>[8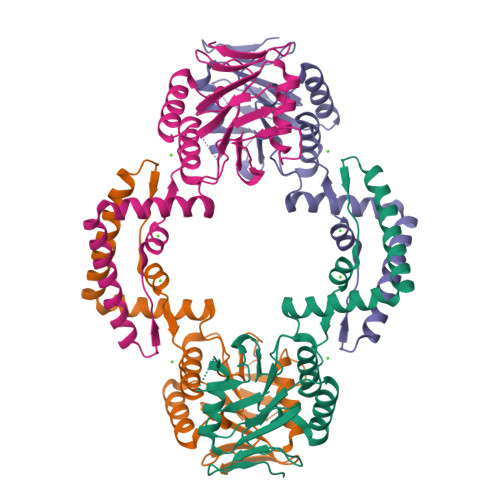x]SMRVNFSLLEEPIEIEKATFLTIKDVQSFAHLVKLIYQYDGENELKLFDAQQKGLKPTELFVVTDILGYDVNSAATLKLIYGDLEAQLNDKPEVKSMIEKLTGTISQLIGYELLEHEMDLEEDGIIVQELFKALGIKIETTSDTIFEKVMEITQVHRYLSKKKLLIFINACTYLTEDEVQQVVEYISLNNVDVLFLEQRVVQNRFQYILDENFYLSYEKA(1S,3S,4E)-3-({3-hydroxy-2-methyl-5-[(phosphonooxy)methyl]pyridin-4-yl}methyl)-4-iminocyclopentane-1-carboxylic 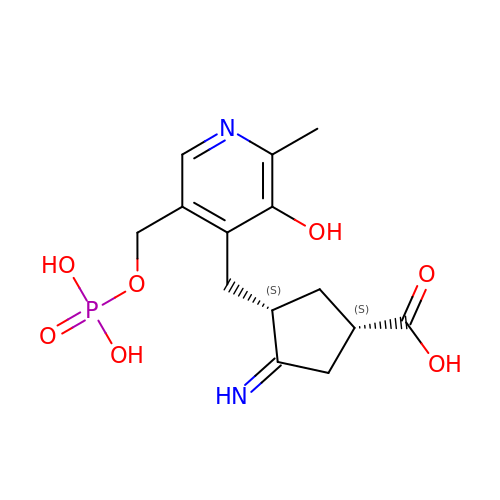acid | C14 H19 N2 O7 P | CTOWFYUCLIAQOJ-QEPOKVMRSA-N> GSMEYEWKPDEQGLQQILQLLKESQS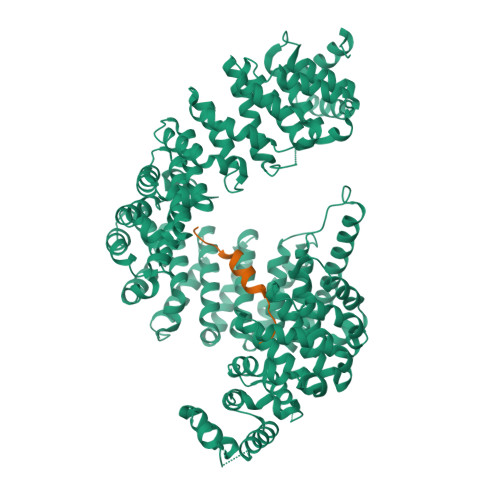PDTTIQRTVQQKLEQLNQYPDFNNYLIFVLTKLKSEDEPTRSLSGLILKNNVKAHFQNFPNGVTDFIKSECLNNIGDSSPLIRATVGILITTIASKGELQNWPDLLPKLCSLLDSEDYNTCEGAFGALQKICEDSAEILDSDVLDRPLNIMIPKFLQFFKHSSPKIRSHAVACVNQFIISRTQALMLHIDSFIENLFALAGDEEPEVRKNVCRALVMLLEVRMDRLLPHMHNIVEYMLQRTQDQDENVALEACEFWLTLAEQPICKDVLVRHLPKLIPVLVNGMKYSDIDIILLKGDVEEDETIPDSEQDIRGGSGGSGDTISDWNLRKCSAAALDVLANVYRDELLPHILPLLKELLFHHEWVVKESGILVLGAIAEGCMQGMIPYLPELIPHLIQCLSDKKALVRSITCWTLSRYAHWVVSQPPDTYLKPLMTELLKRILDSNKRVQEAACSAFATLEEEACTELVPYLAYILDTLVFAFSKYQHKNLLILYDAIGTLADSVGHHLNKPEYIQMLMPPLIQKWNMLKDEDKDLFPLLECLSSVATALQSGFLPYCEPVYQRCVNLVQKTLAQAMLNNAQPDQYEAPDKDFMIVALDLLSGLAEGLGGNIEQLVARSNILTLMYQCMQDKMPEVRQSSFALLGDLTKACFQHVKPCIADFMPILGTNLNPEFISVCNNATWAIGEISIQMGIEMQPYIPMVLHQLVEIINRPNTPKTLLENTAITIGRLGYVCPQEVAPMLQQFIRPWCTSLRNIRDNEEKDSAFRGICTMISVNPSGVIQDFIFFCDAVASWINPKDDLRDMFCKILHGFKNQVGDENWRRFSDQFPLPLKERLAAFYGV;> GSGGGPGGSHMGGNYGDDRRGGRGGYDRGGYRGRGGDRGGFRGGRGGGDRGGFGPGKMDSRGEHRQDRRERPY> ENQKEYF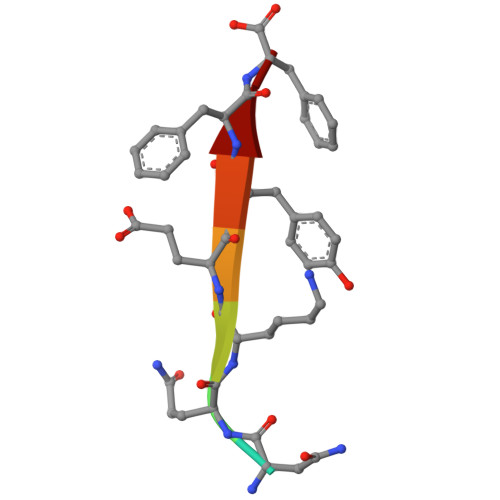F We have previously shown that the dedicated assembly chaperone Acl4 recognizes nascent RpL4, facilitates its nuclear import, and releases RpL4 on engaging RpL18 at the pre-ribosome. Moreover, Acl4 is required for the soluble expression of newly synthesized RpL4 and for the protection of RpL4 from the Tom1-dependent cellular degradation machinery. Whereas, unprotected RpL4 is targeted by the E3-ubiquitin ligase Tom1 for proteasome-dependent degradation, interactions with Acl4 and Kap104 sequester Tom1 ubiquitination sites in the RpL4 loop and extension. Thus, ribosome assembly chaperones can serve dual functions by facilitating nuclear import while simultaneously protecting unassembled ribosomal proteins from the cellular degradation machinery.

Moreover, we determined the 3.0-Å resolution crystal structure of the karyopherin transport factor Kap104 in complex with the eukaryote specific RpL4 extension. RpL4EXT harbours a canonical basic phenylalanine-tyrosine nuclear localization signal (PY-NLS) and alanine mutagenesis confirmed that all canonical elements of its consensus sequence are critical for the Kap104–RpL4EXT interaction. To explore whether RpL4EXT residues Lys310 and Lys340 are protected by Kap104 in a similar fashion, we determined the crystal structure of Kap104 in complex with RpL4EXT to 3.0 Å resolution. The Kap104·RpL4EXT structure revealed that the PY-NLS of RpL4EXT engages the concave surface of Kap104 in the same binding mode as previously established for other PY-NLS sequences. RpL4LOOP residue Lys56 along with RpL4EXT residues Lys310 and Lys340 were identified as Tom1 recognition sites, which were ubiquitinated in the absence of Acl4 and Kap104. Upon Kap104 binding to RpL4EXT and formation of a nuclear import complex both Tom1-modification sites of RpL4EXT are sequestered by the concave Kap104 surface, consistent with our previous protection results of an in vitro Tom1 ubiquitination assay. Our structural and biochemical analysis demonstrates that the RpL4 extension possesses overlapping binding sites for a second Acl4 copy and Kap104. Indeed, in a competition experiment Kap104 replaced the RpL4EXT-bound Acl4 copy to form an Acl4·RpL4·Kap104 complex. Kap104 replaces one Acl4 copy and shuttles Acl4·RpL4 across the nuclear envelope. Once in the nucleus, Kap104 releases RpL4EXT on RanGTP binding allowing the rebinding of a second Acl4 copy from the nuclear Acl4 pool.

> MEYEWKPDEQGLQQILQLLKESQSPDTTIQRTVQQKLEQLNQYPDFNNYLIFVLTKLKSEDEPTRSLSGLILKNNVKAHFQNFPNGVTDFIKSECLNNIGDSSPLIRATVGILITTIASKGELQNWPDLLPKLCSLLDSEDYNTCEGAFGALQKICEDSAEILDSDVLDRPLNIMIPKFLQFFKHSSPKIRSHAVACVNQFIISRTQALMLHIDSFIENLFALAGDEEPEVRKNVCRALVMLLEVRMDRLLPHMHNIVEYMLQRTQDQDENVALEACEFWLTLAEQPICKDVLVRHLPKLIPVLVNGMKYSDIDIILLKGDVEEDETIPDSEQDIGGSGGSGDDTISDWNLRKCSAAALDVLANVYRDELLPHILPLLKELLFHHEWVVKESGILVLGAIAEGCMQGMIPYLPELIPHLIQCLSDKKALVRSITCWTLSRYAHWVVSQPPDTYLKPLMTELLKRILDSNKRVQEAACSAFATLEEEACTELVPYLAYILDTLVFAFSKYQHKNLLILYDAIGTLADSVGHHLNKPEYIQMLMPPLIQKWNMLKDEDKDLFPLLECLSSVATALQSGFLPYCEPVYQRCVNLVQKTLAQAMLNNAQPDQYEAPDKDFMIVALDLLSGLAEGLGGNIEQLVARSNILTLMYQCMQDKMPEVRQSSFALLGDLTKACFQHVKPCIADFMPILGTNLNPEFISVCNNATWAIGEISIQMGIEMQPYIPMVLHQLVEIINRPNTPKTLLENTAITIGRLGYVCPQEVAPMLQQFIRPWCTSLRNIRDNEEKDSAFRGICTMISVNPSGVIQDFIFFCDAVASWINPKDDLRDMFCKILHGFKNQVGDENWRRFSDQFPLPLKERLAAFYGV;> SRTKRACVQKKNPLRNKQIMLRLNPY>[12x]MTNKISSSDNLSNAVSATDDNASRTPNLNRRALVGGGVGLAARGALASGLQAATLPAGASQVPTTPAGRPMPYAIRPMPEDRRFGYAIVGLGKYALNQILPGFAGCQHSRIEALVSGNAEKAKIVAAEYGVDPRKIYDYSNFDKIAKDPKIDAVYIILPNSLHAEFAIRAFKAGKHVMCEKPMATSVADCQRMIDAAKAANKKLMIGYRCHYDPMNRAAVKLIRENQLGKLGMVTTDN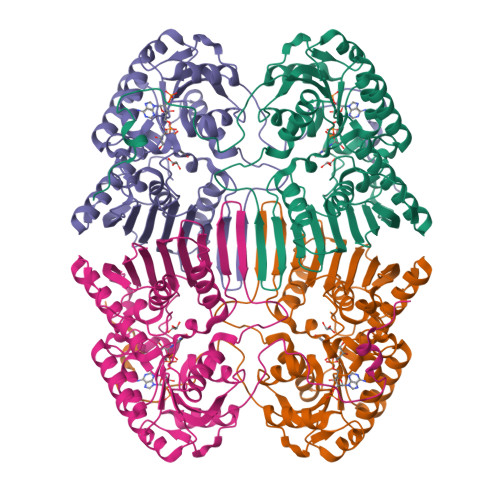SDVMDQNDPAQQWRLRRELAGGGSLMDIGIYGLNGTRYLLGEEPIEVRAYTYSDPNDERFVEVEDRIIWQMRFRSGALSHGASSYSTTTTSRFSVQGDKAVLLMDPATGYYQNLISVQTPGHANQSMMPQFIMPANNQFSAQLDHLAEAVINNKPVRSPGEEGMQDVRLIQAIYEAARTGRPVNTDWGYVRQGGY>MKHTLPDLPFDYADLEPVISHEIMQLHHQKHHATYVNNLNQIEEKLHEAVSKGNLKEAIALQPALKFNGGGHINHSIFWTNLAKDGGEPSKELMDTIKRDFGSLDNLQKRLSDITIAVQGSGWGWLGYCKKDKILKIA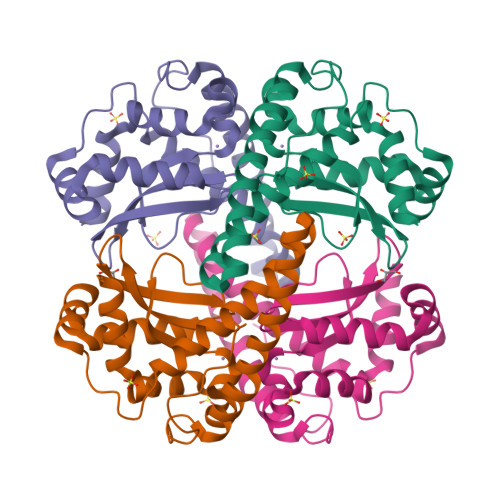TCANHDPLEGMVPLFGIDVWEHAYYLQYKNVRPDYVHAIWKIANWKNISERFANARQ[2x]>ARSEESARSQVQVHAPVVAARLRNIWPKFPKWLHEAPLAVAWEVTRLFMHCKVDLEDESLGLKYDPSWSTARDVTDIWKTLYRLDAFRGKPFPEKPPNDVFVTAMTGNFESKGSAVVLSAVLDYNPDNSPTAPLYLVKLKPLMFEQGCRLTRRFGPDRFFEILIPSPTSTSPSVPPVVS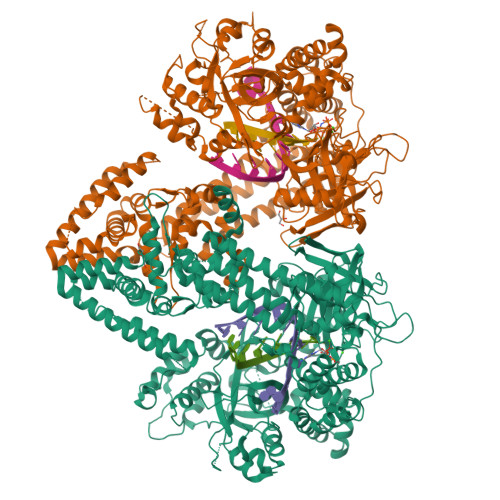KQPGAVEEVIQWLTMGQHSLVGRQWRAFFAKDAGYRKPLREFQLRAEDPKPIIKERVHFFAETGITFRPDVFKTRSVVPAEEPVEQRTEFKVSQMLDWLLQLDNNTWQPHLKLFSRIQLGLSKTYAIMTLEPHQIRHHKTDLLSPSGTGEVMNDGVGRMSRSVAKRIRDVLGLGDVPSAVQGRFGSAKGMWVIDVDDTGDEDWIETYPSQRKWECDFVDKHQRTLEVRSVASELKSAGLNLQLLPVLEDRARDKVKMRQAIGDRLINDLQRQFSEQKHALNRPVEFRQWVYESYSSRATRVSHGRVPFLAGLPDSQEETLNFLMNSGFDPKKQKYLQDIAWDLQKRKCDTLKSKLNIRVGRSAYIYMIADFWGVLEENEVHVGFSSKFRDEEESFTLLSDCDVLVARSPAHFPSDIQRVRAVFKPELHSLKDVIIFSTKGDVPLAKKLSGGDYDGDMAWVCWDPEIVDGFVNAEMPLEPDLSRYLKKDKTTFKQLMASHGTGSAAKEQTTYDMIQKSFHFALQPNFLGMCTNYKERLCYINNSVSNKPAIILSSLVGNLVDQSKQGIVFNEASWAQLRRELLGGALSLPDPMYKSDSWLGRGEPTHIIDYLKFSIARPAIDKELEAFHNAMKAAKDTEDGAHFWDPDLASYYTFFKEISDKSRSSALLFTTLKNRIGEVEKEYGRLVKNKEMRDSKDPYPVRVNQVYEKWCAITPEAMDKSGANYDSKVIRLLELSFLADREMNTWALLRASTAFKLYYHKSPKFVWQMAGRQLAYIKAQMTSRPGEGAPALMTAFMYAGLMPDKKFTKQYVARLEGDGSEYPDPEVYEVLGDDDFDGIGFTGNGDY[2x]4-chloro-N-cyclopentyl-1-methyl-1H-pyrazole-3-carboxamide | C10 H14 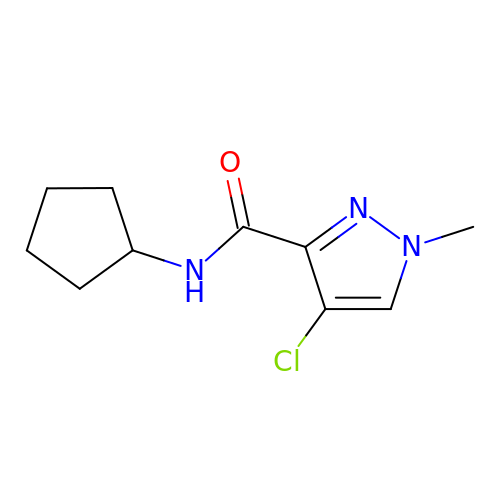Cl N3 O | AEWMHZKRUKXXFH-UHFFFAOYSA-N> XSITKTELDGILPLVARGKVRDIYEVDAGTLLFVATDRISAYDVIMENSIPEKGILLTKLSEFWFKFLSNDVRNHLVDIAPGKTIFDYLPAKLSEPKYKTQLEDRSLLVHKHKLIPLEVIVRGYITGSAWKEYVKTGTVHGLKQPQGLKESQEFPEPIFTPSTKAEQGEHDENISPAQAAELVGEDLSRRVAELAVKLYSKCKDYAKEKGIIIADTKF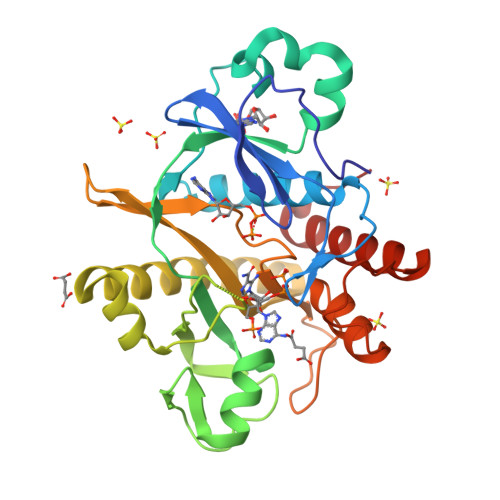EFGIDEKTNEIILVDEVLTPDSSRFWNGASYKVGESQDSYDKQFLRDWLTANKLNGVNGVKMPQDIVDRTRAKYIEAYETLTGSKWSH> MKHHHHHHSAGLEVLFQGPDSMQNQGSVSQGALNMRDQQAAAAENVTPERVWALWNEGNLFSLSLAQLQGFLSRCGVRTDPAAKKAAVVRQVEEYLHSKDTTVKGGGQGAASPQQHQQHGQQGGYGRWNQASVMQPETLLDLSQAGFYEGAANMVPKAFQLLVSDTAPDVVVSRVNTTAFPGFPSNTECYTLGASEKDVAIRSRYSKVLQWCCLNMSNLQMDGELYVDFGKLLLKPSVMRKNRRIVSSYTLQQRLQVNHPYTWVPTLPESCLSKIQEQFLQPEGFAPIGKGVQLTYSGTIKRSKDQLHVDLDNKGKVLAVNSAWVNLQTAWCTHAKGPDVRLLLRSRPPIRRQDVELFASTPIIKLADDDVADVLPPEHGQLVYLSEDETRLFE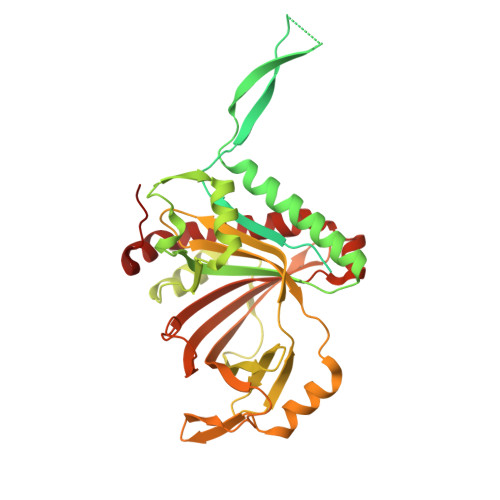RVSDRGVTITVREVKRQPLIILRDEEEDPRVEYSLSAHIPANAAKATDVRAVGLTAFELAGRLAGLVAEDFVREYGCEAKL>MKTPEDCTGLADIREAIDRIDLDIVQALGRRMDYVKAASRFKASEAAIPAPERVAAMLPERARWAEENGLDAPFVEGLFAQIIHWYIAEQIKYWRQTRG[2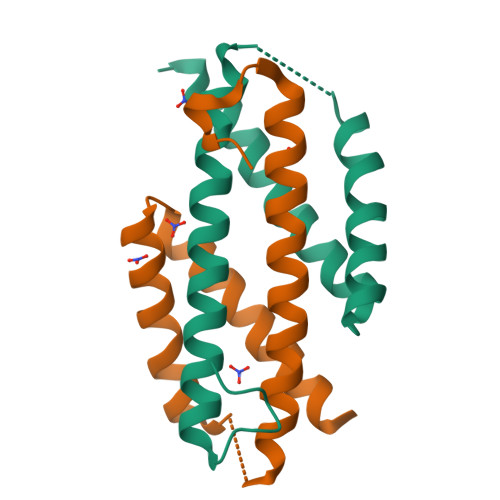x]>[2x]MGSSHHHHHHSQGSEFMDPLSPPLCTLPPGPEPPRFVCYCEGEESGEGDRGGFNLYVTDAAELWSTCFTPDSLAALKARFGLSAAEDITPRFRAACE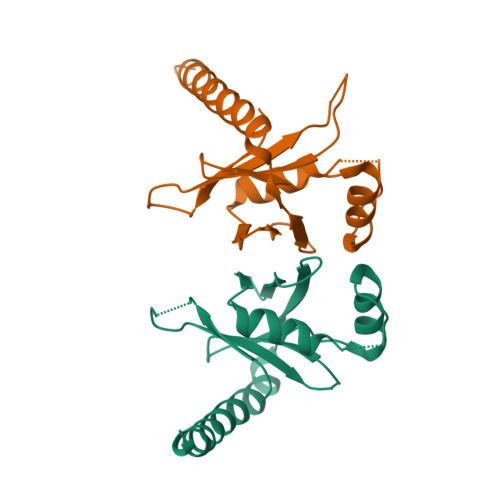QQAVALTLQEDRASLTLSGGPSALAFDLSKVPGPEAAPRLRALTLGLAKRVWSLERRLAAAEET Reversal of PARylation is predominantly carried out by poly(ADP-ribose) glycohydrolase (PARG) in nucleus and cytosol, whereas ADP-ribosylhydrolase 3 (ARH3) may play a role in mitochondrial PAR degradation. PARG comprises an N-terminal regulatory/targeting domain and a C-terminal catalytic domain. The mouse PARG catalytic domain has a bean-shaped structure, with the active site in a deep cleft in the middle on the abdominal side.

Under a new crystallization condition, we obtained a second crystal form (space group P21212) successfully soaked in ADPr and ADP-HPD, and solved the complex structures by molecular replacement. ADPr or ADP-HPD binds to the active site cleft of mPARG. The signature catalytic loop (GGGVTGAGLVQEE) interacts with the ribose ring of ADPr or the pyrrolidine ring of the ADP-HPD. Residue Glu748 forms a hydrogen bond with the 2″-OH, while the key catalytic residue Glu749 side chain carboxyl group is very close to the 1′-OH of the ADPr or the C1″ of the ADP-HPD. Residue Asn733 forms another hydrogen bond with 3″-OH to recognize the ligand. The second conserved glycine rich loop (GCGAFGGD) interacts with the diphosphate group of the ADPr or ADP-HPD. Residue Phe868 side chain is also in close contact with the ribose ring of ADPr or the pyrrolidine ring of ADP-HPD. On the adenine-linked ribose side, the adenine ring interacts extensively with mPARG. Our PARG structure in complex with ADPr and ADP-HPD suggests that mouse PARG uses a very similar mechanism. In contrast to bacterial PARG in which the 2′-OH of the adenine-linked ribose is buried, the same 2′-OH group in mouse PARG structure is exposed to the solvent, which would allow mPARG to bind (n+1) ADPr.

>[3x]GNLPPEKKWLGTPIEEMRKMPRCGIHLPSLRPSASHTVTVRVDLLRAGEVPKPFPTHYKDLWDNKHVKMPCSEQNLYPVEDENGERTAGSRWELIQTALLNKFTRPQNLKDAILKYNVAYSKKWDFTALVDFWDKVLEEAEAQHLYQSILPDMVKIALCLPNICTQPIPLLKQKMNHSVTMSQEQIASLLANAFFCTFPRRNAKMKSEYSSYPDINFNRLFEGRSSRKPEKLKTLFCYFRRVTEKKPTGLVTFTRQSLEDFPEWERCEKPLTRLHVTYEGTIEGNGRGMLQVDFANRFVGGGVTGAGLVQEEIRFLINPELIVSRLFTEVLDHNECLIITGTEQYSEYTGYAETYRWARSHEDGSEKDDWQRRCTEIVAIDALHFRRYLDQFVPEKVRRELNKAYCGFLRPGVPSENLSAVATGNWGCGAFGGDARLKALIQILAAAAAERDVVYFTFGDSELMRDIYSMHTFLTERKLDVGKVYKLLLRYYNEECRNCSTPGPDIKLYPFIYHAVESSAET>[16x]GSFSAADVYVPDEWEVAREKITMSRELGQGSFGMVYEGVAKGVVKDEPETRVAIKTVNEAASMRERIEFLNEASVMKEFNCHHVVRLLGVVSQGQPTLVIMELMTRGDLKSYLRSLRPEMENNPVLAPPSLSKMIQMAGEIADGMA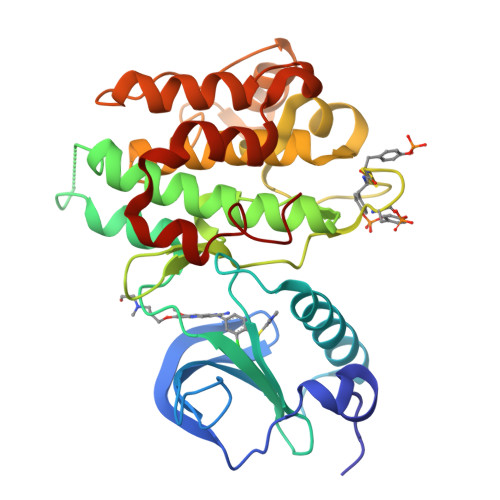YLNANKFVHRDLAARNCMVAEDFTVKIGDFGMTRDIYETDYYRKGGKGLLPVRWMSPESLKDGVFTTYSDVWSFGVVLWEIATLAEQPYQGLSNEQVLRFVMEGGLLDKPDNCPDMLFELMRMCWQYNPKMRPSFLEIISSIKEEMEPGFREVSFYYSEENK4-AMINOBENZOIC ACID | C7 H7 N O2 | 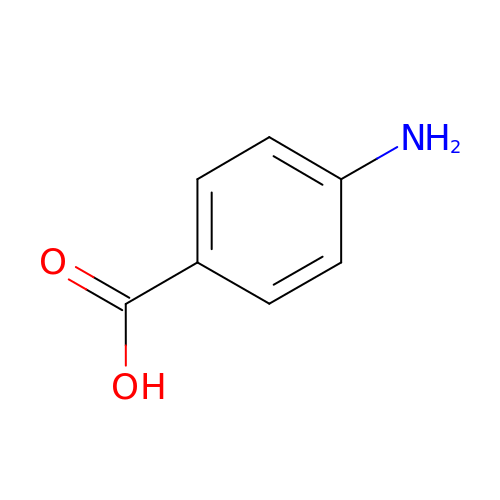ALYNCZNDIQEVRV-UHFFFAOYSA-N> APVLENRRARHDYEILETYEAGIALKGTEVKSLRAGKVDFTGSFARFEDGELYLENLYIAPYEKGSYANVDPRRKRKLLLHKHELRRLLGKVEQKGLTL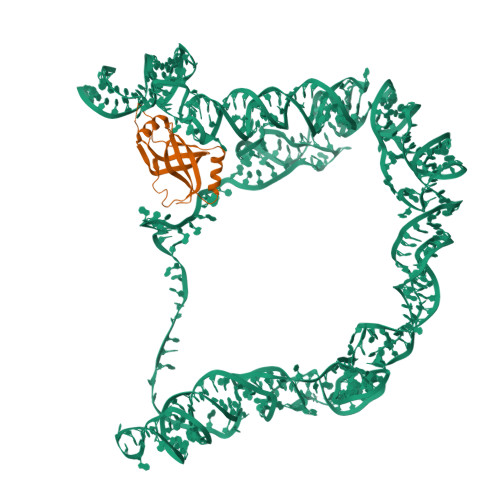VPLKIYFNERGYAKVLLGLARGK> MGHHHHHHMELEGLTALVTGGTSGIGLESARLMAAEGADVVITGRDAQRGEQAAADIGHGARFVQADLGDLDSVADLAAQAPDVDILVNNAGIYPQASTFDQDVAGFQQLFDTNVRGTYFLVAAAAKGMVARGHGSIVNITTLAAHKGFPGTSVYGATKAALESLTRTWAAEFGANGVRVNSVSPGPTRTPTTLEQLGDFIDDVAAGLPLRRTAAPEEIAQAVLFLASPRASFVTG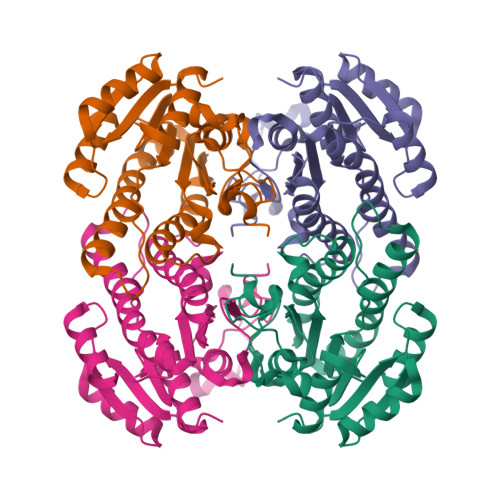STLYVDGGGYAV N-(3-acetylphenyl)morpholine-4-carboxamide | C13 H16 N2 O3 | 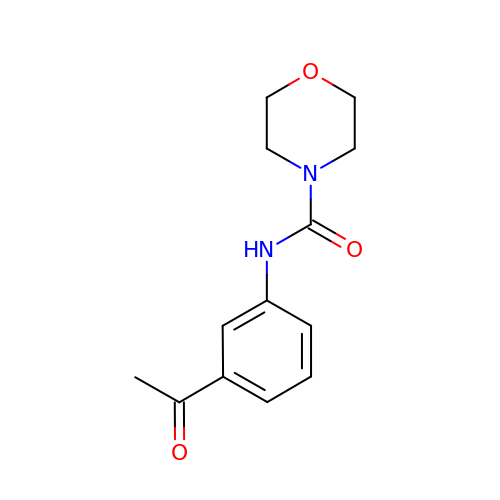GFGGXIIHWJXKMZ-UHFFFAOYSA-N> MAHHHHHHMSEVANEASRRRTFAIISHPDAGKTTLTEKLLLFGGAIQMAGSVKGRKAARHATSDWMALEKERGISVTSSVMQFPYEDKIVNLLDTPGHADFGEDTYRVLTAVDSALMVIDVAKGVEERTIKLMEVCRLRDTPIMTFINKLDREGKDPIELLDEVETVLGIQCAPVTWPIGMGQRLKGVVHLLTGEVHLYEPGRNFTRQDSTIFPSIDAPGLAEKIGAQMLADLRDELELVQGASHPFDLEAYR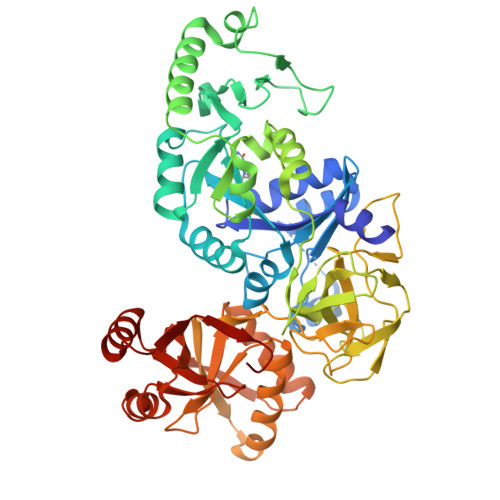AGKQTPVFFGSGVNNFGVQPLLDFFVEHAPSPQARSTTGREIAPEENKLTGFVFKIQANMDPQHRDRVAFMRVCSGRFSAGMKTFHVRTGKEMKLANALTFMASDREIAAEAWPGDVIGIHNHGTISIGDTFTEGEAVTFTGIPNFAPELFRRARLRDPLKLKQLQKGLAQLSEEGATQFFRPLTSNDLILGAVGVLQFDVAAYRLKDEYGVEATFEPVSVTTARWVHCSNEKKLEEFREKNALNLALDAAGHLVYLAPTRVNLQLAQERSPDVRFSATREAAHTVSVG> AASQSTPWGIKAIYNNSN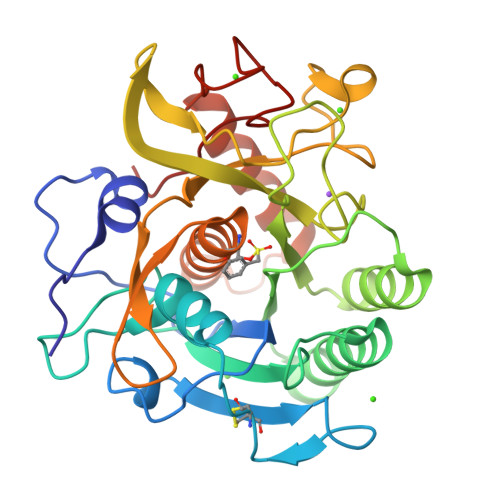LTSTSGGAGINIAVLDTGVNTNHPDLSNNVEQCKDFTVGTNFTDNSCTDRQGHGTHVAGSALANGGTGSGVYGVAPEADLWAYKVLGDDGSGYADDIAEAIRHAGDQATALNTKVVINMSLGSSGESSLITNAVDYAYDKGVLIIAAAGNSGPKPGSIGYPGALVNAVAVAALENTIQNGTYRVADFSSRGHKRTAGDYVIQKGDVEISAPGAAVYSTWFDGGYATISGTSMASPHAAGLAAKIWAQSPAASNVDVRGELQTRASVNDILSGNSAGSGDDIASGFGFAKVQ The adhesion G protein–coupled receptor CD97 and its ligand complement decay-accelerating factor CD55 are important binding partners in the human immune system. Adhesion GPCRs are characterized by variable tandem adhesion domains followed by a common GPCR autoproteolysis-inducing (GAIN) domain at the extracellular region and a canonical seven-transmembrane (7TM) domain at the C-terminal region. CD55 is a GPI-linked membrane protein with four short consensus repeat (SCR) domains at the N terminus. CD55 regulates the complement cascade by inactivating the C3 convertases and plays a critical role in inflammation and pathogen defense.

Herein, we report the structure of the adhesive domains of the CD97–CD55 complex as determined at 3.19 Å resolution by X-ray crystallography. The CD55 and CD97 bind roughly antiparallel to each other involving each N-terminal tandem domains. Structures of CD55 and CD97 in the complex superimposed closely with prior monomeric structures, with a Cα r.m.s.d. of 0.9 to 2.1 Å and 1.1 to 1.2, respectively, suggesting no conformational change is needed during binding. In CD97 or EMR2, EGF2 and EGF5 each bind a calcium ion in the N-terminal tip, which contributes to rigidity within the interface of EGF1–EGF2 or EGF2–EGF5. Our complex structure reveals two N-glycosylation sites in CD97 (Asn-38 and Asn-108) and one N-glycosylation site in CD55 (Asn-95), but none of these carbohydrates are involved in the CD97–CD55 interactions. The preeminent interactions of CD97–CD55 come from the EGF2–SCR1/SCR2 interface in the middle region, which buries a total surface area of 1278 Å2 and contains six pairs of hydrogen bonds. In the third interface of EGF5–SCR1, Val-137 of EGF5 inserts into a joint hydrophobic pocket formed by SCR1 residues Val-60, Lys-76, Val-79, Ile-80, and Leu-82 and EGF2 residue Phe-79. In CD97, the Pro-71 and its preceding residue Thr-70 adopt a cis-peptide conformation, allowing the Thr-70 to flip its backbone and form a hydrogen bond to Glu-99 in the CD55 SCR2 domain. The majority of the interactions of CD55 with CD97 come from this SCR1–SCR2 pair, including six of the seven total hydrogen bonds between the two proteins. The overall architecture of the CD55–CD97 binding mode together with structural details leads to a shearing stretch geometry, which is known to resist force applied to the protein interface.

> QDSRGCARWCPQNSSCVNATACRCNPGFSSFSEIITTPTETCDDINECATPSKVSCGKFSDCWNTEGSYDCVCSPGYEPVSGAKTFKNESENTCQDVDECSSGQHQCDSSTVCFNTVGSYSCRCRPGWKPRHGIPNNQKDTVCED;> SDCGLPPDVPNAQPALEGRTSFPEDTVITYKCEESFVKIPGEKDSVICLKGSQWSDIEEFCNRSCEVPTRLNSASLKQPYITQNYFPVGTVVEYECRPGYRREPSLSPKLTCLQNLKWSTAVEFCKKKSCPNPGEIRNGQIDVPGGILFGATISFSCNTGYKLFGSTSSFCLISGSSVQWSDPLPECREIYCPAPPQIDNGIIQGERDHYGYRQSVTYACNKGFTMIGEHSIYCTVNNDEGEWSGPPPECR> TDPRAKWVPQDNDIQACDYWRHCSIDGNICDCSGGSLTNCPPGTKLATASWVASCYNPTDGQSYLIAYRDCCG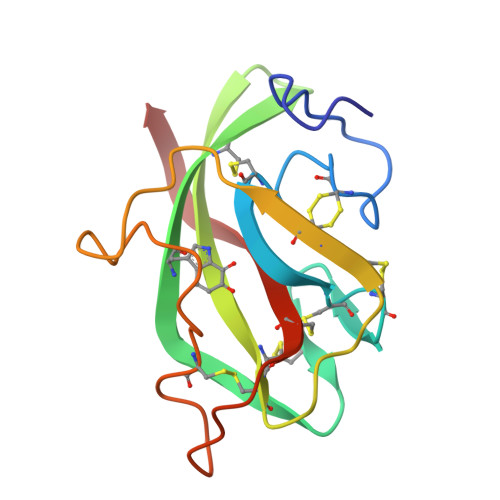YNVSGRCPCLNTEGELPVYRPEFANDIIWCFGAEDDAMTYHCTISPIVGKAS Signaling through RET plays essential regulatory roles in the development of the nervous system and kidney. Glia cell line-derived growth factor (GDNF), Neurturin (NRTN), Artemin (ARTN) and Persephin are four ligands that induce dimerization of RET through assembling 2:2:2 ternary complexes with RET and the co-receptors GDNF receptor-α family proteins (GFRα1–4). Here, we report the cryo-EM structures of four extracellular 2:2:2 ligand/co-receptor/RET complexes, including GDF15/GFRAL/RET, GDNF/GFRα1/RET, NRTN/GFRα2/RET and ARTN/GFRα3/RET, at near-atomic resolution. The structures show that the extracellular region of RET adopts a ‘C-clamp’ shape, which is stabilized by extensive inter-domain interactions as well as binding of calcium ion at multiple sites.

The reconstruction of the GDNF/GFRα1/RET complex reached lower resolution (4.4 Å) due to preferred orientation of particles. The structure of the intact RET extracellular region in complex with GDNF and GFRα1 has been determined at low resolution by negative-stain electron microscopy (EM), showing an overall batwing-like shape in which the two wing-shaped RET molecules are tethered together by the dimeric GDNF/GFRα1 complex in the middle, and suggesting that the CRD is important for the dimerization and activation of RET. All four complexes show the same batwing-like architecture as shown in the previously reported negative-stain EM structure of the GDNF/GRFα1/RET, with the dimeric ligands located at the center connecting the two wings formed together by RET and the co-receptors. The segments in GFRα1, GFRα2 and GFRα3 corresponding to the helix-loop-helix-loop motif in GFRAL are much shorter and adopt extended loop conformations. As a result, interfaces I in GFRα1/RET, GFRα2/RET and GFRα3/RET are much smaller (buried surface areas less than 700 Å2) and likely weaker than that in GFRAL/RET (buried surface area ~ 1500 Å2). Interfaces II of GFRα1, GFRα2 and GFRα3 with RET (buried surface areas ~ 730–1010 Å2) however are more extensive than that in GFRAL/RET (buried surface areas ~ 680 Å2), which may partially compensate for their weaker interfaces I. The D1 domain of the co-receptors is invisible in the 3D reconstructions of GDF15/GFRAL/RET, GDNF/GFRα1/RET, and ARTN/GFRα3/RET, suggesting that it is not involved in the binding to either RET or the ligands in these three complexes. However, there are large differences in the angle between the two wings of the batwing-shaped complexes, which mainly originate from the different conformations of the ligand dimers and their different interfaces with the co-receptors. This angle in the GDF15/GFRAL/RET complex (~60°) is much more acute than that in the complexes of GDNF/GFRα1/RET (130°), NRTN/GFRα2/RET (105°) and ARTN/GFRα3/RET (108°).

>[2x]SPDKQMAVLPRRERNRQAAAANPENSRGKGRRGQRGKNRGCVLTAIHLNVTDLGLGYETKEELIFRYCSGSCDAAETTYDKILKNLSRNRRLVSDKVGQACCRPIAFDDDLSFLDDNLVYHILRKHSAKRCGCI;>DRLDCVKASDQCLKEQSCSTKYRTLRQCVAGKETNFSLASGLEAKDECRSAMEALKQKSLYNCRCKRGMKKEKNCLRIYWSMYQSLQGNDLLEDSPYEPVNSRLSDIFRVVPFISDVFQQVEHIPKGNNCLDAAKACNLDDICKKYRSAYITPCTTSVSNDVCNRRKCHKALRQFFDKVPAKHSYGMLFCSCRDIACTERRRQTIVPVCSYEEREKPNCLNLQDSCKTNYICRSRLADFFTNCQPESRSVSSCLKENYADCLLAYSGLIGTVMTPNYIDSSSLSVAPWCDCSNSGNDLEECLKFLNFFKDNTCLKNAIQAFGNGSDVTVWQPAFPVQTTTATTTTALRVKNKPLGPAGSENEIPTHVLPPCANLQAQKLKSNVSGNTHLCISNGNYEKEGLGGTHHHHHHHH[2x];>LYFSRDAYWEKLYVDQAAGTPLLYVHALRDAPEEVPSFRLGQHLYGTYRTRLHENNWICIQEDTGLLYLNRSLDHSSWEKLSVRNHGFPLLTVYLKVFLSPTSLREGECQWPGCARVYFSFFNTSFPACSSLKPRELCFPETRPSFRIRENRPPGTFHQFRLLPVQFLCPNISVAYRLLEGEGLPFRCAPDSLEVSTRWALDREQREKYELVAVCTVHAGAREEVVMVPFPVTVYDEDDSAPTFPAGVDTASAVVEFKRKEDTVVATLRVFDADVVPASGELVRRYTSTLLPGDTWAQQTFRVEHWPNETSVQANGSFVRATVHDYRLVLNRNLSISENRTMQLAVLVNDSDFQGPGAGVLLLHFNVSVLPVSLHLPSTYSLSVSRRARRFAQIGKVCVENCQAFSGINVQYKLHSSGANCSTLGVVTSAEDTSGILFVNDTKALRRPKCAELHYMVVATDQQTSRQAQAQLLVTVEGSYVAEEAGCPLSCAVSKRRLECEECGGLGSPTGRCEWRQGDGKGITRNFSTCSPSTKTCPDGHCDVVETQDINICPQDCLRGSIVGGHEPGEPRGIKAGYGTCNCFPEEEKCFCEPEDIQDPLCDELCRGTHHHHHHHH[2x]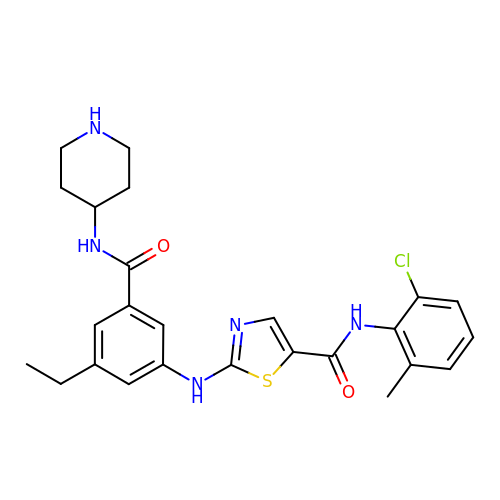~{N}-(2-chloranyl-6-methyl-phenyl)-2-[[3-ethyl-5-(piperidin-4-ylcarbamoyl)phenyl]amino]-1,3-thiazole-5-carboxamide | C25 H28 Cl N5 O2 S | AVCRYIXULVHLPG-UHFFFAOYSA-N>[4x]STMKFMA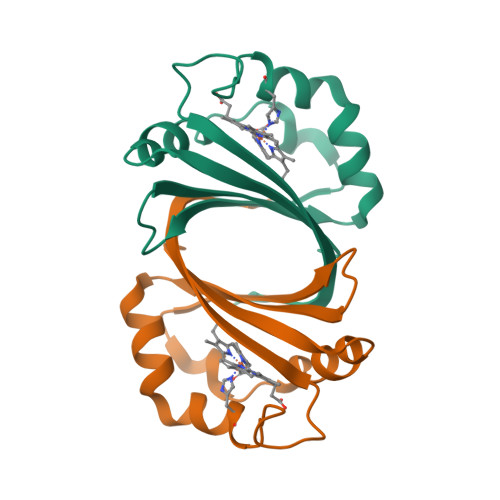EARLTLTKGTAKDIIERFYTRHGIETLEGFDGMFVTQTLEQEDFDEVKILTVWKSKQAFTDWLKSDVFKAAHKHVRSKNEDESSPIINNKVITYDIGYSYMK>[4x]PKYTIVDKETCIACGA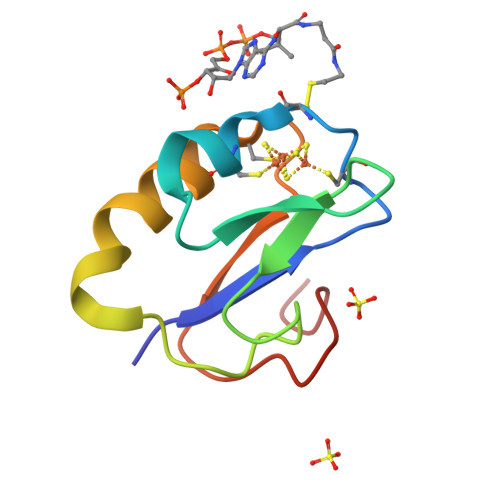CGAAAPDIYDYDEDGIAYVTLDDNQGIVEVPDILIDDMMDAFEGCPTDSIKVADEPFDGDPNKFE>MVKSSGTERKERMDTSSLM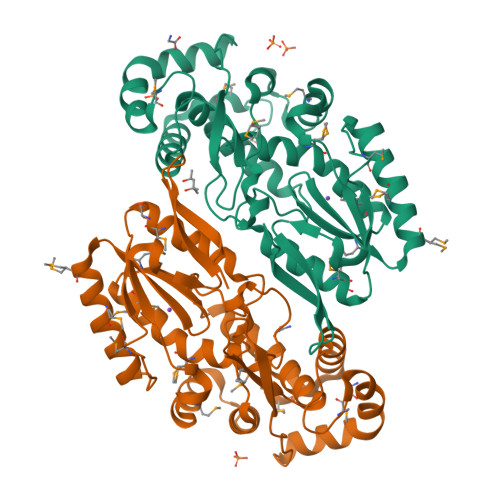EQILSNDNLNRAYLQVVRNKGAEGVDGMKYTELKEYLAKNGEIIKEQLRIRKYKPQPVRRVEIPKPDGGVRNLGVPTVTDRFIQQAIAQVLTPIYEEQFHDHSYGFRPNRCAQQAILTALDMMNDGNDWIVDIDLEKFFDTVNHDKLMTIIGRTIKDGDVISIVRKYLVSGIMIDDEYEDSIVGTPQGGNLSPLLANIMLNELDKEMEKRGLNFVRYADDCIIMVGSEMSANRVMRNISRFIEEKLGLKVNMTKSKVDRPRGIKYLGFGFYYDTSAQQFKAKPHAK[2x]>[4x]GPLGSENDLGITAVALYDYQAAGDDEISFDPDDIITNIEMIDDGWWRGVCK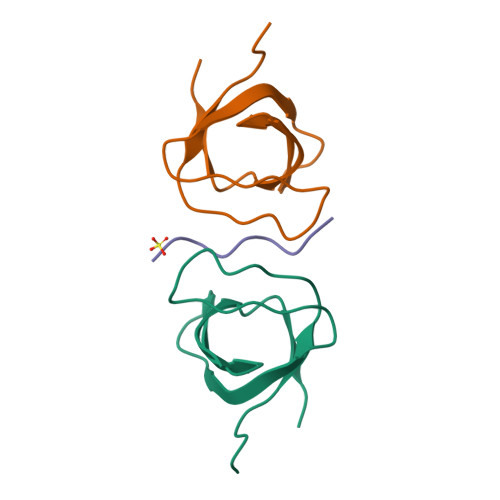GRYGLFPANYVELRQ;>SKKRPPPPPPGHKRT[2x]>[4x]GSMPLLLDDGDPKAQTGFDLSTATTLFWRPVPVHVKQQDREDVLEELTFRILTGVAKQNHNLRILRIHISSDSDLFFL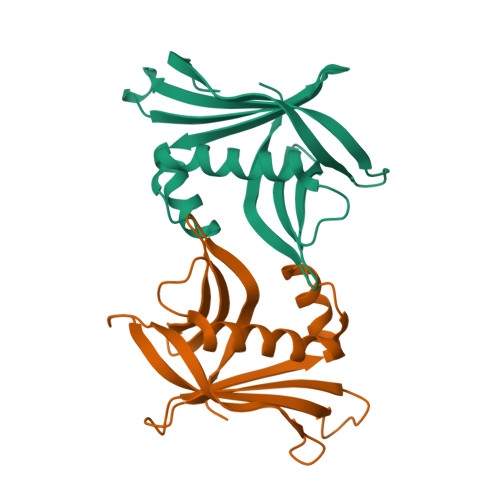HTLEVSEEDFQSLKNDQGILVDFASFPGKIISLLEKCILAQPGDSPRFQAVLTIRGGESVFKIVEINDWKQLPHITLAFRPGN> RLQRLIQLISPHVDDCDARCLVDLCWAVWGFRGAPDVVEPLLNRMASVVVRRENAFTPKQLGTIAFTFSWFRGAPTDTVADFVLAECVKLLPEMEPFHVTLLFGSLRRMRRLNRDVANLMIEKLTDDIDRFTSDDVVGVLRALAANSITRGFLLRRVATLVFDNLDSFKPKQLASVLNS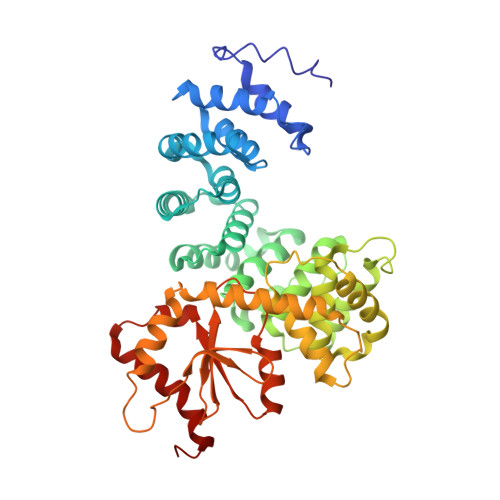LTLLRFLTVENGEELFSCLSGSLSELPAASIAEILEALTILNFPRPEVVRTCLDLLAEKNGLISQGSWVRDHMIIAAHAVIQFQLYDKNPVVKPLLEELFRSRVNSSRTQHRVEEVIHALDLEKASPRVDVPPYWRAMIDQANREEQARLEHSGLQNELTLVLDSLRGKFQLQIQKNQQAGPYSVQFLDDETKICIEIDYPCCRTPHIIKARHLKQLGYHYLLVDCWQWRRLRSEAEQTVFLKQLLSGPLLEVGRLEG In conclusion, we have resolved the full-length structure of a ZntB transporter, a member of the CorA MIT family. ZntB is a distant homologue of CorA proteins, which are well-characterized magnesium (and cobalt) channels. By combining all available data from us and other groups, we conclude that ZntB is a zinc importer that is driven by a proton gradient. Each protomer of ZntB consists of a large N-terminal cytoplasmic domain folded into an αβα motif.

The apo structure of ZntB was obtained by single-particle cryo-electron microscopy (cryo-EM) using n-dodecyl-β-d-maltopyranoside (DDM)-solubilized and purified E. coli ZntB (EcZntB) (pre-treated with ethylenediaminetetraacetic acid (EDTA)) and resolved at an overall resolution of 4.2 Å. Analysis of the substrate translocation pore revealed a wider profile in ZntB than in the magnesium channels TmCorA and MjCorA. All three proteins have short extracellular loops between TM1 and TM2, where the family signature motif GxN that forms the selectivity filter is located. Our work on ZntB shows that the mechanism cannot be extrapolated to other members of the family, because even after an extensive treatment with EDTA ZntB maintained its symmetrical pentameric state. In contrast to stringent removal of Mg2+ from CorA channels, the depletion of Zn2+ from ZntB is likely to be physiologically relevant because intracellular concentrations of free Zn2+ are extremely low (i.e., in the pM–fM range). Therefore the symmetrical structure of ZntB may better represent the apo state than the asymmetrical structure of CorA. Whereas our structure was obtained in the absence of Zn2+, StZntB was crystallized in the presence of Zn2+. Calculation of the surface potentials revealed dramatic differences between full-length EcZntB and soluble StZntB. The cytoplasmic domain of full length EcZntB has a strong positive electrostatic surface potential (resembling VpZntB), whereas the potential in the isolated domain of StZntB is negative. Furthermore, the shape of the internal pore between two forms is different possibly resembling two conformational states.

>[5x]MEAIKGSDVNVPDAVFAWMLDGRGGVKPLENTDVIDEAHPCWLHLNYVHHDSAQWLATTPLLPNNVRDALAGESTRPRVSRLGEGTLITLRCINGSTDERPDQLVAMRVYMDGRLIVSTRQRKVLALDDVVSDLEEGTGPTDCGGWLVDVCDALTDHSSEFIEQLHDKIIDLEDNLLDQQIPPRGFLALLRKQLIVMRRYMAPQRDVYARLASERLPWMSDDQRRRMQDIADRLGRGLDEIDACIARTGVMADEIAQVMQENLARRTYTMSLMAMVFLPSTFLTGLFGVNLGGIPGGGWQFGFSIFCILLVVLIGGVALWLHRSKWL>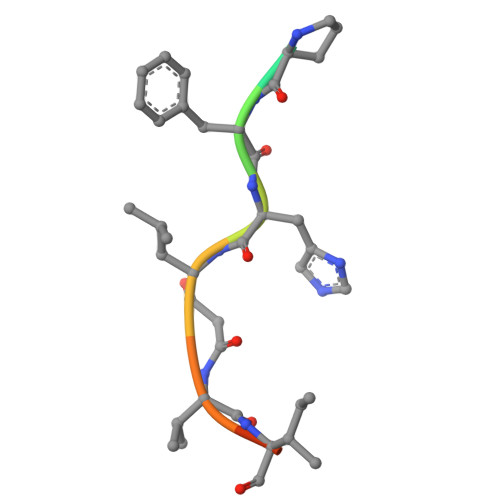 PHPFHXVIHK>[2x]GSHGMRSVSGQVVCVTGAGGFIASWLVKILLEKG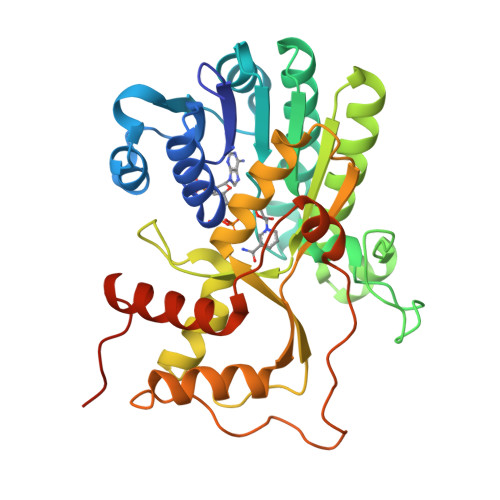YTVRGTVRNPDDPKNGHLRELEGAKERLTLCKADLLDYQSLREAINGCDGVFHTASPVTDDPEQMVEPAVIGTKNVINAAAEANVRRVVFTSSIGAVYMDPNRDPETVVDETCWSDPDFCKNTKNWYCYGKMVAEQAAWEEAKEKGVDLVVINPVLVQGPLLQTTVNASVLHILKYLTGSAKTYANSVQAYVDVKDVALAHILLYETPEASGRYLCAESVLHRGDVVEILSKFFPEYPIPTKCSDVTKPRVKPYKFSNQKLKDLGLEFTPVKQCLYETVKSLQEKGHLPIPTQKDEPIIRIQP>[10x]MASTTRLVNDRKQLEQQVKDDARILADARGLNITTVANDSATGGQAIRNVGPNDEATIKALDNVIKQIEALSVIVNRSEKADDAQILGPNTYKQLLEHLFSPEENVYILLPIQAYTGGVIDRRDASFSNFAYSIASKLMMELSAATHNKIFTDYTRIAASALGPEISTEGMPLFSLIESLELTEAETSRLPVIQDSMVIQKSTATVGNAQQGISTINIKRVPFVGSAFQQVIDQLLWEYSTTSLTTKEQRRQRITEMVNDRRIMIQKLTLAEKPQVMRHVTTEINNDLFFKMSPVAQLYIYHLDRAFLDGVGFTPLAEKQQQLQLQLKTNILTANLIRSAINGMNTESNLEVAIKMMQAAQLHRASIEIAFPMNVSLSPEIIVQCFIVWMSIPEQLLSDRSNFIIAAVIWAGFSADDSYADIMRRSARASDRQNYDIIKAALSSRKFKLPRASTTLFDENEPVVRRYQIGRVYAPFPVDRYGSPVYSNCTKVELASDYNAEGFTIRKDDFRALQAVLRIDEDRAADMFTTLRIMISSIPAVWYDAEVVHYPHTAVELEQLAAYGLTGAYPRTNHSVDTIVKTVNNISATYSTIAQMLSTIDLDPTRYGTSESIDKFKIAWENVESVLNMEGNDFVKTIMYAYEDNFPKKDFYMMLKQIASDGQGAHPIAAAIDQLRTIVYREPERFGYIDSVILTHNPDVDTAYNRFFHLHPIVTNQPSNTIKNAQLWNEMRLEQQVEHIKAGPVRIIGPFHVTYNYLSEEEDMPATSHIIMKDNMILNDHLTFNFVKRERRNNKKRVSSFRYKAVEMYVAVRISRFQLEVLRDLHDLVRSRTYLDVSKSPLATTPIRVVEYVR;> MRIMAQRLKELQREIDKKKKERIAEAYLSSVEVTNSSPSLSKQDDALTLPKVSPFLDSTPFTTLHNSLYGQQIHSIDDELAQICKLEYELQTQIADEQITALKHFLTIRTGSPQEIQYVDKEWMKSNQHVPSFLGDVKLMFGDTAGKFRSTSKSVDSIHSITSDVQVTRKKQTRSQIRNSYRVQKKHKVQQPLKPNTLYVYKYKGLPRVVLRFVPKVDTTSNSNSSSASDSKKDKDAFSCDDLSPTWKYILTEAKRAFPDRSYSDCIHPMTWEEWLEENQDHVKVLTQYAHQLDYVTLLQDFNLYVSGGASRVRNIDMSTLPTSINVLDHFELYGDASMKEYVRSGEWYGLLREIEQEGMTVNESEKVFANPDTYVLNVKKYFLRRFQQEIASTGMTPLTDELLNIMFVHWNIIVTAEPKLQVIKDDLLKYYSRYGVDATFDYNMKRSEMTVVTRGHLLAHKVLECALRIVETIYTYDIQDETFKDILIDLGRLIMRDPIYGTTTVRDATTVMKQLMYTQGTQFRRIMFKKYDYSNFNEKLVLKGEQMTNEPPTLLATTHYEEMDKKRIDALIKANQRAGNILSQSSIERCRYTDSLDLVGDANRYFSALTTLEAVAGFASSDLLSGFIDSNESIEFTGTAHLRKLLYHSVREQITTLNTSTVPRPSLPKVLLSSAKDTASASIEPLTFRIYKTTPEYDGESLNLVESTVEMSTRQKKPNLMKAAEILRSTVTTNQEMIISGGTRAVQGGKGARAVYPTKQPYHIAGSLLFHKVDTIVNANKKYRGVSNKYGQGISNAIPHIGVPEIIAVSSDGMAICLALDVSAFDVAQKYTEADIELAMRDGFLDSEISMISGETVLERMNPADLANNLLTNTPPRYKYQTALGDIIILQHDNRSGVPWTGTQNDLVNVSNHHMAYDEYKKRVAELQRQGKISIDVNDKHHIVRVFGDDSTFIMTYDEPPSAEEVHLMCATFVESYQDTAGTLGFAINARKGMIGRYGSEYLKNSAIYGNIKSVNQVKFRGSEKSASYHFGVSEKVSMIRDITDLTITRGCDETRKWKYNLMMLPVDLTTRAGAFRMHNLCSIMTGVGKMYLGGTLNNKLIASYHGSSFGWNFDDNLIKTANSIGAISDSSYDAISTKITNLADFKDSQQRITRDIITSGRLPQHLNRYGKSNILRHILASAAMGPLSQIEKNVNAYNVVMGILNGKLEAPTVLERLNMGFKYVVMSDLKQDDYSPYSCQGLQYRRMLVHWGLNDSRITSFDPKGKLQHLLAKNSQILPIHFDIEFVYRLYLQAGTMGFLQVMSYYQLPDTLTHEMLAAVVALELQLGNDKYAVDMGVYSSQAGQIRINDALMDSIIQHRRGPPLPIIDRTLNRLLLHTYMLMFGLMGKSIDSTKIDPTLSWRAILESNDQRIAQLSELLTAV

A non-turreted virus consisting of a 12-segment dsRNA genome, mud crab reovirus (MCRV), which may belong to a new order of Reovirales, infects the economically important crab Scylla serrata. Like other members of Reovirales, MCRV packages its dsRNA segments and a number of RNA-dependent RNA polymerase (RdRp) inside a double-layered icosahedral capsid. Using cryo-EM, we determined the structure of mud crab reovirus (MCRV), a 12-segmented dsRNA virus that is a putative member of Reovirales in the non-turreted Sedoreoviridae family, to near-atomic resolutions with icosahedral symmetry (3.1 Å) and without imposing icosahedral symmetry (3.4 Å). These structures revealed the organization of the major capsid proteins in two layers: an outer T = 13 layer consisting of VP12 trimers and unique VP11 clamps, and an inner T = 1 layer consisting of VP3 dimers.

Subsequent 3D reconstruction with D5 symmetry imposed resulted in a 3.4 Å resolution map. All copies of the structural proteins in the D5 reconstruction were almost identical to those in the corresponding icosahedral map, with the exception of the well resolved ten RdRps near the ten 5-fold vertices. A hallmark of the MCRV non-icosahedral (C1 and D5) reconstruction is the ten well-resolved RdRp densities located slightly offset (~30 Å) from ten of the twelve icosahedral vertices that are organized with D5 symmetry. The structure of the RdRp revealed a compact, cage-like structure ~75 Å in diameter with an extended protrusion near its innermost surface. The MCRV RdRp can be divided into three domains: an N-terminal domain (residues 1–617), a central polymerase domain (residues 618–1090), and a C-terminal bracelet domain (residues 1091–1422). In addition to the distinctive arrangement, the RdRp of MCRV has two conspicuous structural features: a specific protrusion on the innermost surface of the RdRp, and a long loop that blocks the gap between the thumb and finger subdomains. While the RdRp is located next to the 5-fold vertices, it is offset such that only three of the five VP3AB dimers contact the RdRp. At the N-terminus of VP3A1, residues 59–69 form a loop that facilitates interactions with the RdRp. The extended N-terminus of the VP3A2 interacts with the RdRp, with residues 40–48 forming an anti-parallel β-sheet with the residues 1220–1226 and 1390–1395 of the RdRp. Together, these two unique conformations of N-termini in VP3A essentially bracket opposite sides of the RdRp and likely help anchor the polymerase to the capsid.>[2x]APAGSHMNIKELSLHELCEELKTPAWNAPLTFVGDVGGTSARMGFVREGKNDSVHACVTRYSMKRKDITEIIEFFNEIIELMPASVMKRVKAGVINVPGPVTGGAVGGPFNNLKGIARLSDYPKALFPPGHSAILNDLEAGGFGVLAVSDAHVFSEYFGVMWEGTQWRTCEQEPAGSVIGRGRCLV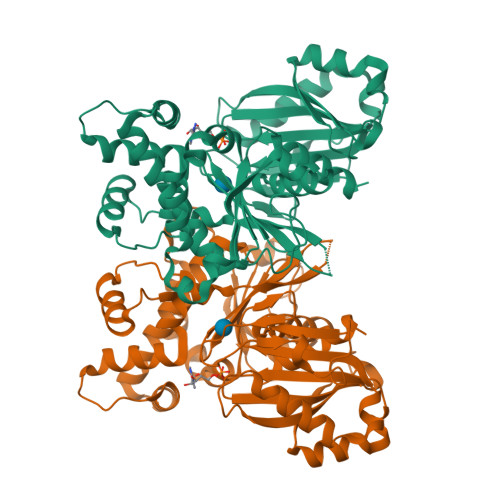LAPGTGLGSSLIYYNPPMNQHIVVPLELGSQTLPMRKDIDYIQTLHAELKLFPNYENMVSGAGLEFHYRQVVRGSRPPCSAGEIAKLASEGDANACKAMKKYHEYLMRVGSEASMALLPLTIVLVGDNIVNNAFFYRNPQNLKEMHHEALNHEMERFGFQSRVSYLRQKKLLNLNLMGCYRCGLDLS>[2x]SEKSEEINEKDLRKKSELQGTALGNLKQIYYYNEKAKTENKESHDQFLQHTIL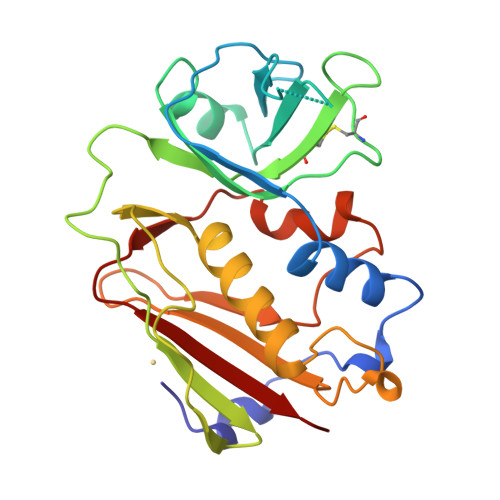FKGFFTDHSWYNDLLVDFDSKDIVDKYKGKKVDLYGAYYGYQCAGGTPNKTACMYGGVTLHDNNRLTEEKKVPINLWLDGKQNTVPLETVKTNKKNVTVQELDLQARRYLQEKYNLYNSDVFDGKVQRGLIVFHTSTEPSVNYDLFGAQGQYSNTLLRIYRDNKTINSENMHIDIYLYTS decyl 2-trimethylazaniumylethyl phosphate | C15 H34 N O4 P | 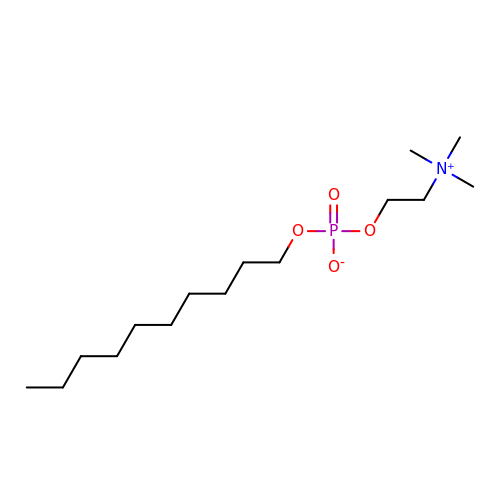VVVDGSCGBGBGFN-UHFFFAOYSA-N2-carbamoylbenzoic 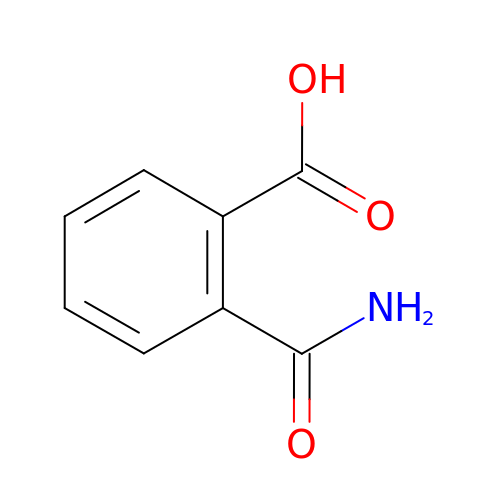acid | C8 H7 N O3 | CYMRPDYINXWJFU-UHFFFAOYSA-N2-[5-(4-methoxyphenyl)-1,2,3,4-tetrazol-2-yl]ethanamine | C10 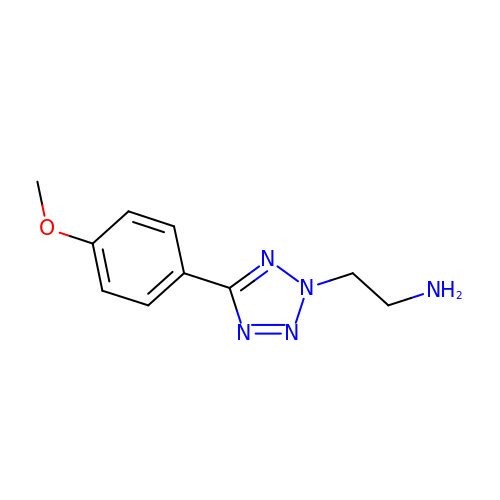H13 N5 O | FHPKDNRSYHKLSG-UHFFFAOYSA-N>MQLKRVAEAKLPTPWGDFLMVGFEELATGHDHVALVYGDISGHTPVLARVHSECLTGDALFSLRCDCGFQLEAALTQIAEEGRGILLYHRQEGRNIGLLNKIRAYALQDQGYDTVEANHQLGFAADERDFTLCADMFKLLGVNEVRLLTNNPKKVEILTEAGINIVERVPLIVGRNPNNEHYLDTKAEKMGHLLNK[2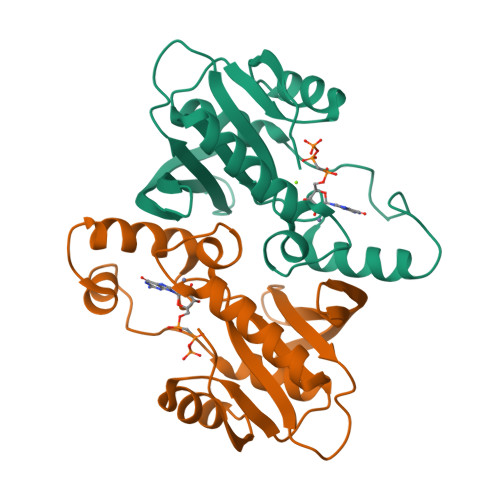x]> MASMTGGQQM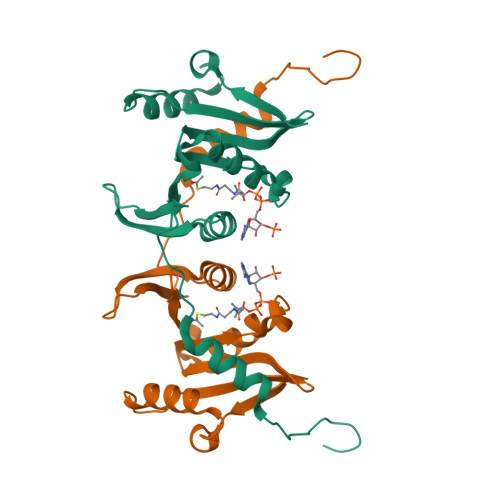GRGSEFELMLVINVVEDKIPANVYPELVEWVRDLNSIREEPIKLTMFVEDDIVRGIMAWEPGHLVYMVVPEESRRGGVGRFMLKYLQQNSDRKHVSCRVHPTNIPALGFFHQQGFQIDRWYIAADGQRYFRMTNYNVISSHTPPEEKLLTHYAESVPIFLSMAEGQFVLEHHHHHH> DAPSALYAPSALVL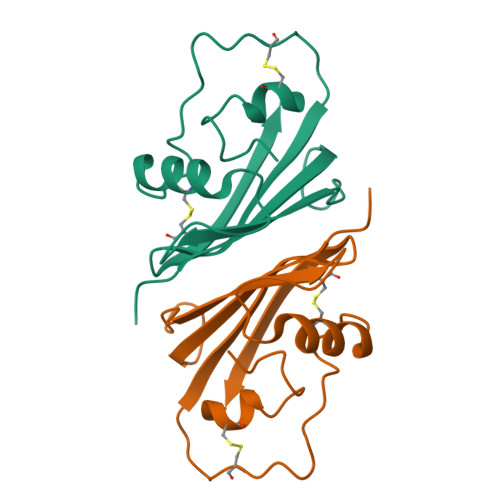TVGKGVSATTAAPERAVTLTCAPGPSGTHPAAGSACADLAAVGGDLNALTRGEDVMCPMVYDPVLLTVDGVWQGKRVSYERVFSNECEMNAHGSSVFAF>KENKKLLCRKCKALACYTADVRVIEESHYTVLGDAFKECFVSRPHPKPKQFSSFEKRAKIFCARQ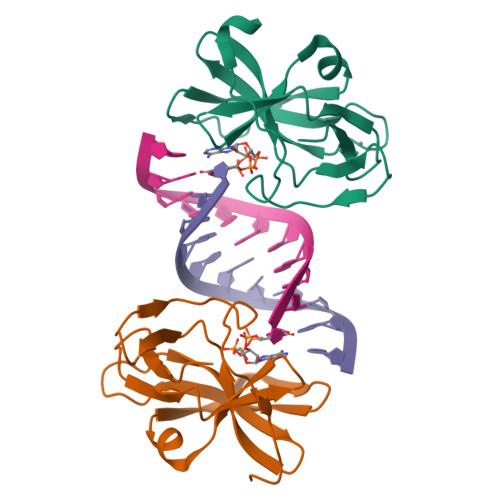NCSHDWGIHVKYKTFEIPVIKIESFVVEDIATGVQTLYSKWKDFHFEKIPFDPAEM[2x]> GSHMAKEEIIWESLSVDVGSQGNPGIVEYKGVDTKTGEVLFEREPIPIGTNNMGEFLAIVHGLRYL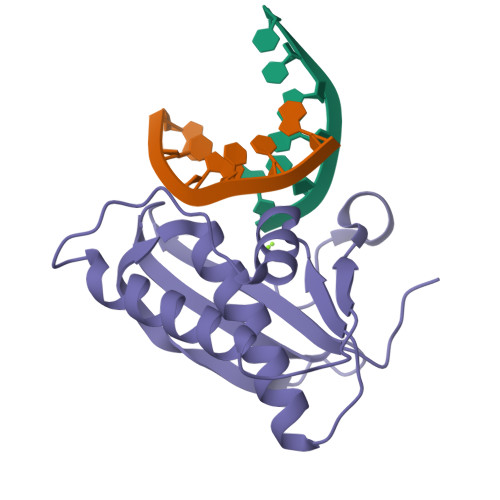KERNSRKPIYSNSQTAIKWVKDKKAKSTLVRNEETALIWKLVDEAEEWLNTHTYETPILKWQTDKWGEIKADYGRK KAT2A is the first identified histone acetyltransferase (HAT) and succinyltransferase. Here, we report that KAT2A can selectively utilize acetyl-CoA, propionyl-CoA, butyryl-CoA, and succinyl-CoA to directly deposit 18 histone acylation hallmarks in nucleosome. By analyzing the co-crystal structures of the catalytic domain of KAT2A in complex with acetyl-CoA, propionyl-CoA, butyryl-CoA, malonyl-CoA, succinyl-CoA, and glutaryl-CoA, we conclude that the alternative substrate-binding pocket of KAT2A and the length and electrostatic features of the acyl chain cooperatively determine the selection of the acyl-CoA substrates by KAT2A. Superimposition analyses revealed that all the studied acyl-CoA molecules fit in the same substrate-binding pocket, surrounded by the sheets of β4 and β6 and the helices of α3 and α5, indicating that all the studied acyl-CoA could potentially be utilized by KAT2A to modify histones.

The studied acyl-CoA molecules can be categorized into 2 types. Acetyl-CoA, propionyl-CoA, and butyryl-CoA are type I CoA molecules without a carboxyl group at the end of the acyl chains. As the acyl chain gets longer, the terminus extends to reach deeper into the binding pocket toward Loop 3, which might occupy the space for the incoming histone lysine residue. KAT2A has an alternative pocket for substrate binding. The propionyl and butyryl chain could flip into the alternative pocket, orienting the reactive carbonyl group of their acyl chain to receive proton transferred from the ε-amino group of the lysine substrate, allowing the covalent modification to occur. Thus, propionyl-CoA and butyryl-CoA can be utilized by KAT2A for histone modifications.

>GIIEFHVIGNSLTPKANRRVLLWLVGLQNVFSHQLPRMPKEYIARLVFDPKHKTLALIKDGRVIGGICFRMFPTQGFTEIVFCAVTSNEQVKGYGTHLMNHLKEYHIKHNILYFLTYADEYAIGYFKKQGFSKDIKVPKSRYLGYIKDYEGATLMECELNPRIPYT[8x]>MTSLFTTADHYHTPLGPDGTPHAFFEALRDEAETTPIGWSEAYGGHWVVAGYKEIQAVIQNTKAFSNKGVTFPRYETGEFELMMAGQDDPVHKKYRQLVAKPFSPEATDLFTEQLRQSTNDLIDARIELGEGDAATWLANEIPARLTAILLGLPPEDGDTYRRWVWAITHVENPEEGAEIFAEL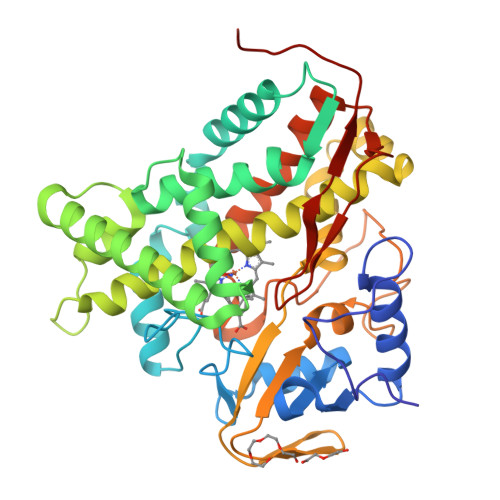VAHARTLIAERRTNPGNDIMSRVIMSKIDGESLSEDDLIGFFTILLLGGIDNTARFLSSVFWRLAWDIELRRRLIAHPELIPNAVDELLRFYGPAMVGRLVTQEVTVGDITMKPGQTAMLWFPIASRDRSAFDSPDNIVIERTPNRHLSLGHGIHRCLGAHLIRVEARVAITEFLKRIPEFSLDPNKECEWLMGQVAGMLHVPIIFPKGKRLSE[2x]>[3x]SNAMTIRFADKADCAAITEIYNHAVLHTAAIWNDRTVDTDNRLAWYEARQLLGYPVLV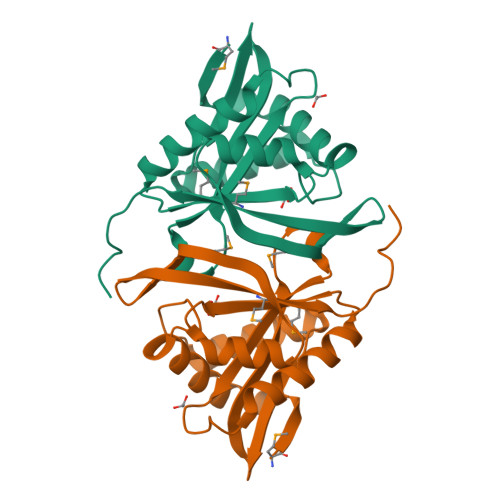SEENGVVTGYASFGDWRSFDGFRYTVEHSVYVHPAHQGKGLGRKLLSRLIDEARRCGKHVMVAGIESQNAASIRLHHSLGFTVTAQMPQVGVKFGRWLDLTFMQLQLDEHAAPDAC> MARKS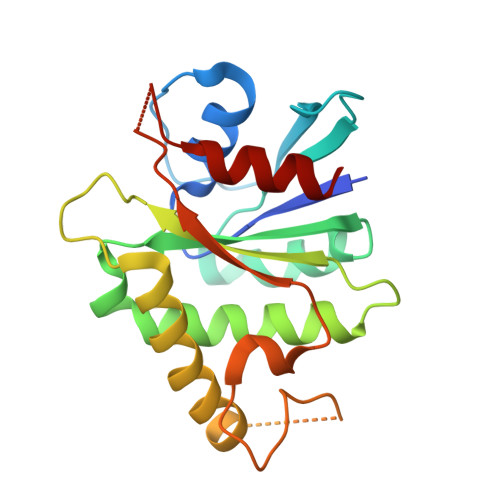SQRAVLFVGLCDSGKTLLFVRLLTGQYRDTQTSITDSSAIYKVNNNRGNSLTLIDLPGHESLRFQLLDRFKSSARAVVFVVDSAAFQREVKDVAEFLYQVLIDSMALKNSPSLLIACNKQDIAMAKSAKLIQQQLEKELNTLRVTRSAAPSTLDSSSTAPAQLGKKGKEFEFSQLPLKVEFLECSAKGGRGDTGSADIQDLEKWLAKIA> MTTSAASQASLPMTTSAA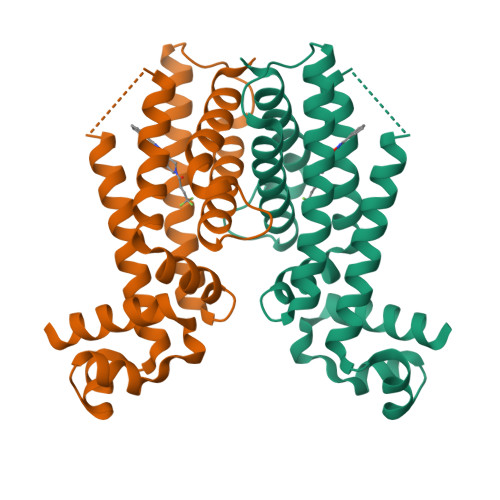SQASLPRGRRTARPSGDDRELAILATAENLLEDRPLADISVDDLAKGAGISRPTFYFYFPSKEAVLLTLLDRVVNQADMALQTLAENPADTDRENMWRTGINVFFETFGSHKAVTRAGQAARATSVEVAELWSTFMQKWIAYTAAVIDAERDRGAAPRTLPAHELATALNLMNERTLFASFAGEQPSVPEARVLDTLVHIWVTSIYGENR In this study, we used solution NMR to investigate the conformational states of small-molecule inhibitors bound to LpxC, an essential metalloamidase that catalyses the deacetylation of UDP-(3-O-acyl)-N-acetylglucosamine during the biosynthesis of lipid A in Gram-negative bacteria. We chose Aquifex aeolicus LpxC (AaLpxC) in the lipid A biosynthetic pathway for structural and dynamics investigation due to its exceptional thermostability, which has enabled both NMR measurements and crystallographic studies (for example, refs 13, 14, 15, 16). Pseudomonas aeruginosa LpxC (PaLpxC) was exploited when co-crystal structures of the desired AaLpxC-inhibitor complexes could not be obtained. We show that these enzyme-bound inhibitors dynamically access alternative, minor conformations in solution in addition to the ligand state observed in the crystal structure.

Taken together, these solution measurement-derived rotamers collectively portray an inhibitor envelope that can accommodate three substitutions at the Cβ position of the threonyl head group. To test this prediction, we merged the two conformations of the threonyl head group and generated Cβ-di-methyl substituted compounds with the third Cβ-substitution containing either a hydroxyl group (LPC-037) or an amino group (LPC-040). Structural analysis of LPC-040 in complex with PaLpxC indeed revealed the anticipated ligand conformation with the two Cβ-substituted methyl groups forming hydrophobic interactions with F180 (F191PaLpxC) and the stem of K227 (K238PaLpxC) and the amino group directed towards solvent accessible space to form a water-mediated hydrogen bond with the backbone carbonyl of F180 (F191PaLpxC). Excitingly, the Cβ-triply substituted compounds LPC-037 and LPC-040 both showed enhanced LpxC inhibition, displaying Ki* values of 14±1 pM and 12±1 pM, respectively.

> MIKQRTLKNIIRATGVGLHSGEKVYLTLKPAPVDTGIVFSRTDLDPVVEIPARAENVGETTMSTTLVKGDVKVDTVEHLLSAMAGLGIDNAYVELSASEVPIMDGSAGPFVFLIQSAGLQEQEAAKKFIRIKREVSVEEGDKRAVFVPFDGFKVSFEIDFDHPVFRGRTQQASVDFSSTSFVKEVSRARTFGFMRDIEYLRSQNLALGGSVENAIVVDENRVLNEDGLRYEDEFVKHKILDAIGDLYLLGNSLIGEFRGFKSGHALNNQLLRTLIADKDAWEVVTFEDARTAPISYMRP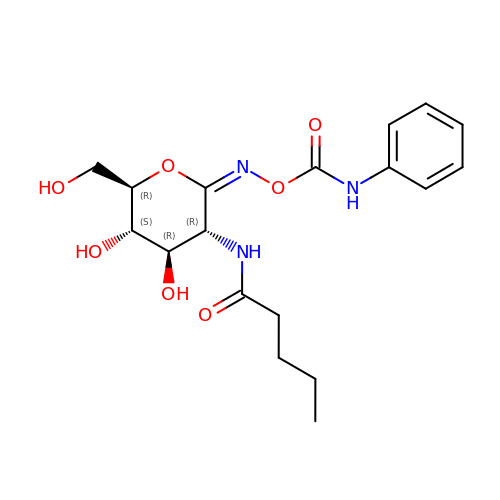[[(3R,4R,5S,6R)-4,5-dihydroxy-6-(hydroxymethyl)-3-(pentanoylamino)oxan-2-ylidene]amino] N-phenylcarbamate | C18 H25 N3 O7 | NUNQIQQEEPOGDJ-JDOAOKHLSA-N> MESYITMNFDKNTAEVGQIIKATVKINKITNFSGYQVNIKYDPTVLQAVNPKTGVAYTNSSLPTSGELLVNEDYGPIVQGVHKISEGILNLSRSYTALDVYRASESPEETGTVAVVGFKALQKKATTVVFEHSVTMPNGIIGTTLFNWYGNRITSGYSVI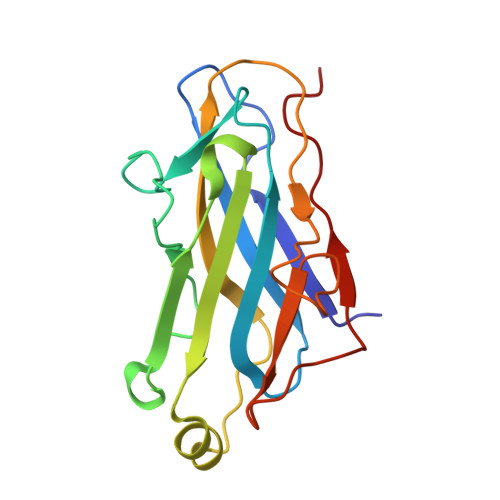QPGEINSE> GGSLTEQDRQLRLLQAQIQRLLEAQSLM

PLK4, and this interaction targets STIL to centrioles. allows homo-multimerisation, the interaction with the PB3 domain of PLK4, or both. structures and interactions of CCDs and PLK4-PB3s in humans and flies. STIL/Ana2, which can then interact with and recruit Sas-6.

characterise this difference, we sought to solve the structure of the HsCCD. coiled-coil dimer of dimers generated by crystallographic symmetry. as an antiparallel dimer of dimers. dimeric form we observe in our structure. concentration and varies between dimeric to nearly tetrameric. reached that of a tetramer at higher concentrations (4000 µM). which is involved in both the dimerisation and PB3 interfaces. and binding to PB3 are likely mutually exclusive. that can readily dissociate to interact with PB3.> GSSHHHHHHSQDPNSSSTKKSAAEASKKPRQKRTATKAYNVTQAFGRRGPEQTQGNFGDQELIRQGTD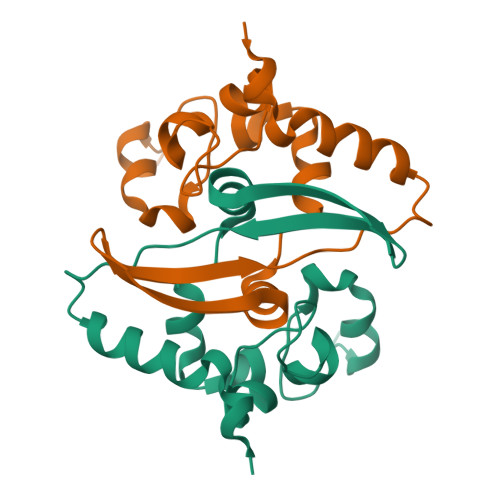YKHWPQIAQFAPSASAFFGMSRIGMEVTPSGTWLTYTGAIKLDDKDPNFKDQVILLNKHIDAYKTFP> HHHHHHQDPEALAAEIGPVKQVSLGEQIDAALAQQGE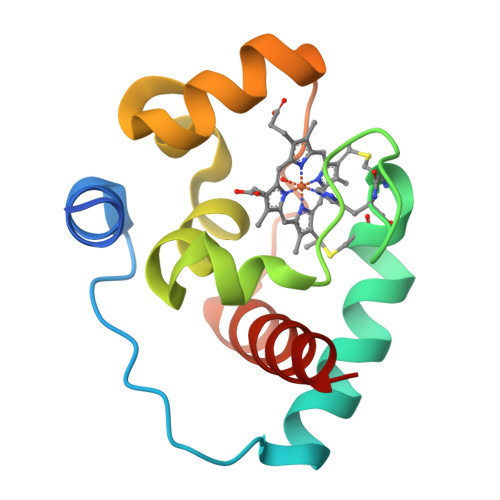QLFNTYCTACHRLDERFIGPALRDVTKRRGPVYIMNTMLNPNGMIQRHPVMKQLVQEYGTMDTDEALSEEQARAILEYLRQVAENQ>MAMRIRIDLPQDEIPAQWYNILPDLPEELPPPQDPTGKSLELLKEVLPSKVLELEFAKERYVKIPDEVLERYLQVGRPTPIIRAKRLEEYLGNNIKIYLKMESYTYTGSHKINSALAHVYYAKLDNAKFVTTETGAGQWGSSVALASALFRMKAHIFMVRTSYYAKPYRKYMMQMYGAEVHPSPSDLTEFGRQLLAKDSNHPGSLGIAISDAVEYAHKNGGKYVVGSVVNSDIMFKTIAGMEAKKQMELIGEDPDYIIGVVGGGSNYAALAYPFLGDELRSGKVRRKYIASGSSEVPKMTKGVYKYDYPDTAKLLPMLKMYTIGSDFVPPPVYAGGLRYHGVAPTLSLLISKGIVQARDYSQEESFKWAKLFSELEGYIPAPETSHALPILAEIAEEAKKSGERKTVLVSFSGHGLLDLGNYASVLFKEKLAA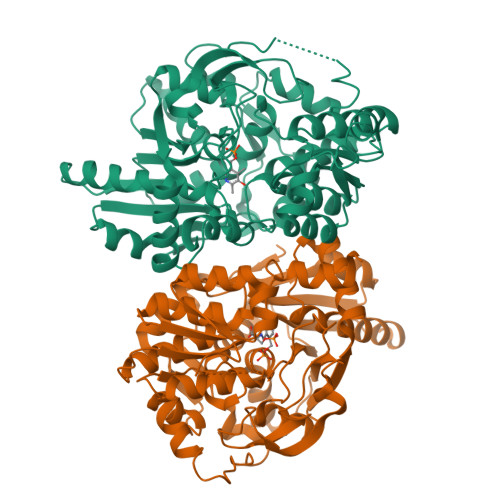ALEHHHHHH[2x]>MGGEVEEPEPQMVLSPLTSAAIFLVVTIDSGGEDTVRDLLSDVASLERAVGFRAQPDGRLSCVTGIGSEAWDRLFSGARPAGLHPFRELDGPVHRAVATPGDLLFHIRASRLDLCFALATEIMGRLRGAVTPQDEVHGFKYFDERDMLGFVAGTENPTGAAARRAVLVGAEDPAFAGGSYAVVQKYLHDIDAWEGLSVEAQERVIGRRKMTDVELSDDVKPADSHVALTSVTGPDGSDLEILRDAMPFGSVGREEFGTYFIGYARTPEVTETMLERMFLGTASAPHDRILDF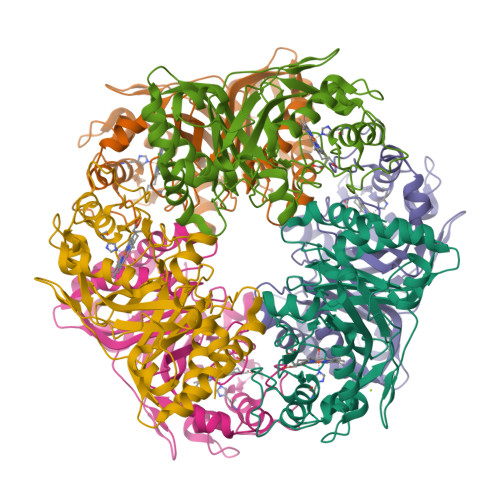STAVTGSLFFTPAADFLEDLSARP[6x]> MVVSIIPQFPDIKVSLALFEQVKNAKEIRSKMSELSTSFAFIDPRLV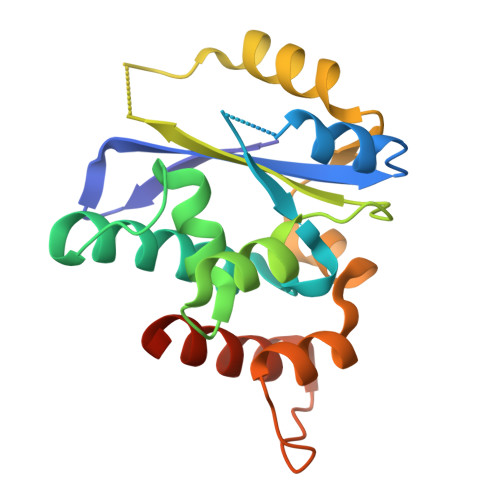CSGEQMYSAIYKTLIEVKYNKMRTRNLNSECVLCLSPTSNISDAFLKFGIKDDSSQLICLKFHTNTDDVDKEQLRTIMTSIVKGQEIEFNDDNLSRFYDEALIRKIYKLSDDFKPQDVNGLSRALVDAIQLRGVHHHHHH>[4x]QVEGKTQKAVCVIYPTQDYKVTGVITFTKSDDGVKVVADLNGLSPGKHGFHIHECGDCSASDGTSAGGHFNPEEKSHGAPMDMSRHIGDLGNITADENGKAHLEYIDKMIVFEGEHSIIGRSMIVHKNEDDLKTQPTGNAGARVACGVIGIGK

Superoxide dismutases and reductases are deployed almost ubiquitously throughout nature to prevent damage to biological molecules by superoxide. They employ redox-active metal cofactors to catalyze the production of molecular oxygen and hydrogen peroxide from superoxide. Crystal structures of a Bacteroidetes bacterium CuZnSOD portray both prokaryotic and eukaryotic characteristics and propose a mechanism for self-catalyzed disulfide maturation. The Group 3 CuZnSODs described here and exemplified by BbCuZnSOD represent an evolutionary intermediary between E-class and P-class enzymes with high eukaryotic sequence identity and E-class homodimerization but P-class functional loops and disulfide configuration.

To investigate, representative Group 2 and 3a enzymes RbCuZnSOD (OUV78940) and BbCuZnSOD (OFX46851) were purified recombinantly from E. coli. This yielded zinc metalated proteins with negligible copper as is the case for human SOD1. Periplasmic bacterial CuZnSODs can follow a different route to maturation as exemplified by the CueP-SodC copper pathway of S. enterica and DsbA-induced oxidative folding of E. coli CuZnSOD. Figure 4 indicates that BbZnSOD is able to form its intrasubunit disulfide bond rapidly in isolation in contrast to SOD1 and RbZnSOD. As the disulfide forms, BbZnSOD transitions from monomers to homodimers indicating BbCuZnSOD forms an E-class homodimer through an interface incorporating the disulfide subloop and that it may follow an autonomous maturation pathway. BbCuZnSOD has a typical eight stranded, anti-parallel, Greek-key β-barrel core structure with two long loops incorporating conserved metal-binding ligands and coordination geometry. The BbCuZnSOD E-class dimer interface area is 747 Å2 comprising N-terminus, C-terminus, and disulfide subloop regions with a PISA score of 1.0 as opposed to 0.2 and 0.3 for human and bovine SOD1, respectively. In addition, each Tyr14 forms two back-bone hydrogen bonds with disulfide bonding Cys146; β-barrel interactions that are conserved in human SOD1. Immediately adjacent to Tyr14 at the loop I N-terminus, Pro15 replaces a glycine which is conserved in 80.5% of eukaryotic CuZnSODs (Gly10, human SOD1). As a result, loop I adopts a conformation shifted toward the disulfide subloop. Crystal structures of this distinctly E-class protein show it includes P-class structural elements positioning several of these bacterial CuZnSODs as an evolutionary stepping-stone between E-class and P-class enzymes.> MADDFGFFSSSESGAPEVAEEDPAAAFLAQQESEIAGIENDEGFGAPAGSQAALAQPGPASGAGPEDMGTTVNGD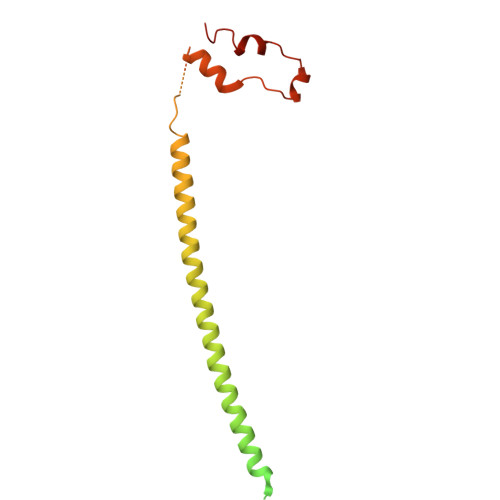VFQDANGPADGYAAIAQADRLTQEPESIRKWREEQRKRLQELDAASKVTEQEWREKAKKDLEEWNQRQSEQVEKNKINNRIADKAFYQQPDADIIGYVASEEAFVKESKEETPGTEWEKVAQLCDFNPKSSKQCKDVSRLRSVLMSLKQTPLSR>[3x]AAYSQGGGKKKVCYYYDGDIGNYYYGQGHPMKPHRIRMTHNLLLNYGLYRKMEIYRPHKATAEEMTKYHSDEYIKFLRSIRPDNMSEYSKQMQRFNVGEDCPVFDGLFEFCQLSTGGSVAGAVKLNRQQTDMAVNWAGGLHHAKKSEASGFCYVNDIVLAILELLKYHQRVLYIDIDIHHGDGVEEAFYTTDRVMTVSFHKYGEYFPGTGDLRDIGAGKGKYYAVNFPMRDGIDDESYGQIFKPIISKVMEMYQPSAVVLQCGADSLSGDRLGCFNLTVKGHAKCVEVVKTFNLPLLMLGGGGYTIRNVARCWTYETAVALDCEIPNELPYNDYFEYFGPDFKLHISPSNMTNQNTPEYMEKIKQRLFENLRMLPHAPGVQMQAI;>XNPEQKWG[3x]

To address this challenge, we develop a computational “anchor extension” methodology for targeting protein interfaces by extending a peptide chain around a non-canonical amino acid residue anchor. To test our approach using a well characterized model system, we design cyclic peptides that inhibit histone deacetylases 2 and 6 (HDAC2 and HDAC6) with enhanced potency compared to the original anchor (IC50 values of 9.1 and 4.4 nM for the best binders compared to 5.4 and 0.6 µM for the anchor, respectively). SHA can coordinate to the zinc ion in the active site of HDACs. In all the crystal structures we obtained, the thiol functional group of SHA coordinates the catalytic Zn2+ ion with a Zn2+– S separation of 2.3 Å in a distorted tetrahedral geometry reminiscent of that observed for the inhibitor Largazole.

Our first computational method (design method 1) started with docking structured cyclic-peptide scaffolds onto SHA and re-designing the residues in the interface to improve binding. Tens of thousands of conformers were generated for each of the 100 peptides, their energies were evaluated, and those designs for which the designed target structure had the lowest energy were selected for downstream analysis. From the previous pool, five peptides with the greatest in silico predicted affinities were tested for HDAC2 inhibition in vitro, the best of which (des1.1.0) demonstrated an IC50 value of 289 nM. The crystal structure of this design in complex with HDAC2 revealed two distinct binding modes and peptide conformations in the three protein chains of the asymmetric unit, suggesting flexibility of the peptide as well as presence of iso-energetic binding conformations. In two of the protein chains of the asymmetric unit (chains B and C), the peptide conformation was very similar to the design model, but the observed binding mode to HDAC2 differed from that of the design model. This binding orientation interacts with several water molecules through backbone-mediated hydrogen bonds. Rosetta-guided mutational scanning successfully stabilized the binding mode observed in the crystal structure (confirmed by structures of variants Lys4→Glu and Pro3→hydroxy-Pro) but failed to significantly improve affinity or selectivity.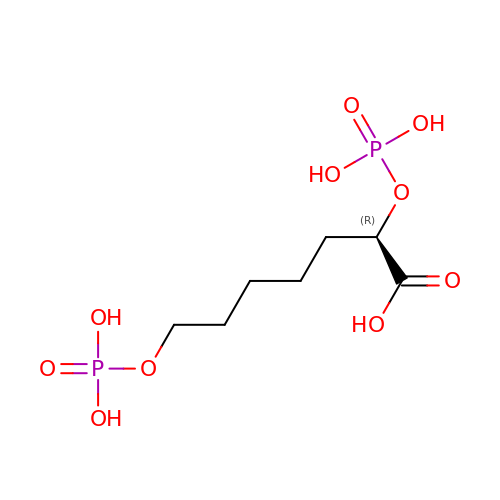(2R)-2,7-bis(phosphonooxy)heptanoic acid | C7 H16 O10 P2 | OZYHUBGACYJJJF-ZCFIWIBFSA-N> CGGRARVREYSRAELVIGTLCRVRVYSKRPAAEVHAALEEVFTLLQQQEMVLSANRDDSALAALNAQAGSAPVVVDRSLYALLERALFFAEKSGGAFNPALGAVVKLWNI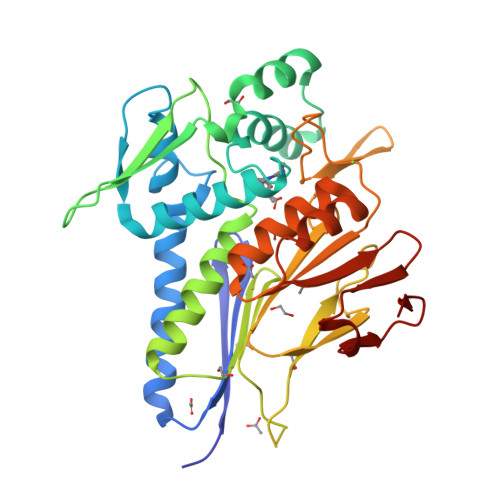GFDRAAVPDPDALKEALTRCDFRQVHLRAGVSVGAPHTVQLAQAGMQLDLGAIAKGFLADKIVQLLTAHALDSALVDLGGNIFALGLKYGDVRSAAAQRLEWNVGIRDPHGTGQKPALVVSVRDCSVVTSGAYERFFERDGVRYHHIIDPVTGFPAHTDVDSVSIFAPRSTDAAALATACFVLGYEKSCALLREFPGVDALFIFPDKRVRASAGIVDRVRVLDARFVLER>GPEIKDYWYTENEITHLLTAQLDEKKFSVQPAITFRNTALTEEMLKDYTAKGEEKNKILAEVQETIKIANLIPDKEERALMLGDAKKREEILKLSDAEREKLKNDLLRGGEAQQQINEDILNRATKDIKDNGKEAAVIPIEMGYGHWTVLVAKYDKKDNQIILTFNDSLGNSINYDGQKLPKLIDKTLGNLPN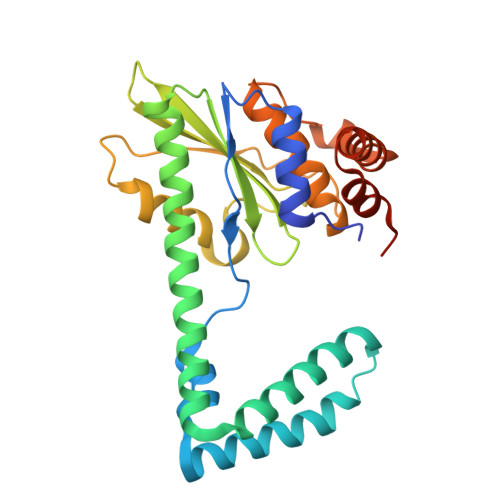KPIIIDEQTKQQTDQSACGVFTVDNGIKIAKGQAILSTEESKGEKGLRLREHHAQILTDAMFKQDAQWIRQQMKTNNNAPD[2x]> GPHMARKFFVGG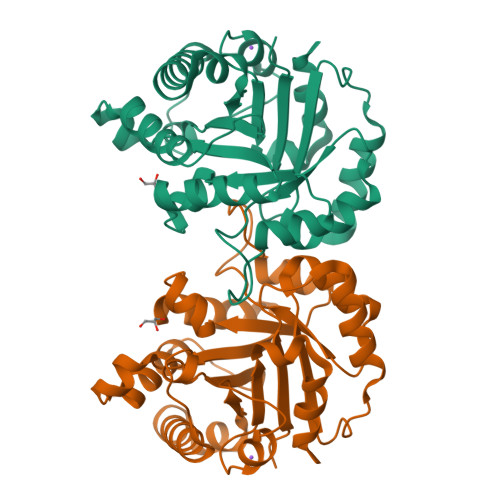NWKDNGTAEEVKKIVNTLNEAQVPSQDVVEVVVSPPYVFLPLVKSTLRSDFFVAAQNCWVKKGGAFTGEVSAEMLVNLDIPWVILGHSERRAILNESSEFVGDKVAYALAQGLKVIACVGETLEEREAGSTMDVVAAQTKAIADRVTNWSNVVIAYEPVWAIGTGKVASPAQAQEVHDELRKWLAKNVSADVAATTRIIYGGSVNGGNCKELGGQADVDGFLVGGASLKPEFIDIIKAAEVKKSA> MGSSHHHHHHTGGTHPAVRVADLLQHINQMKTAEGYGFKQEYESFFEGWDATKKKDKVKGSRQEPMPAYDRHRVKLHPMLGDPSADYINANYIDGYHRSNHFIATQGPKPEMVYDFWRMVWQEHCSSIVMITKLVEVGRVKCSRYWPEDSDTYGDIKIMLVKTETLAEYVVRTFALERRGYSARHEVRQFHFTAWPEHGVPYHATGLLAFIRRVKASTPPDAGPIVIHCSAGTGRTGCYIVLDVMLDMAECEGVVDIYNCVKTLCSRRVNMIQTEEQYIFIHDAILEACLCGETTIP

PTPRU is a member of the R2B receptor family, which includes PTPRK, PTPRM and PTPRT, characterised by large extracellular domains that mediate homophilic interactions and tandem intracellular PTP domains. PTPRU possesses evolutionarily conserved sequence changes to key catalytic motifs including non-canonical WPD (WPE) and pTyr recognition loop sequences (GSRQ rather than KNRY), as well as a unique threonine in the PTP loop. Here, we demonstrate through biochemical and structural studies that PTPRU is unique amongst the receptor-linked protein tyrosine phosphatases (RPTPs) in possessing two pseudophosphatase domains. Despite lacking catalytic activity, PTPRU can recruit substrates of catalytically active paralogs supporting a model where PTPRU functions as a scaffold to compete for binding to protein substrates.

The overall fold of PTPRU-D1 closely resembles related phosphatase domains (RMSD of 1.0 Å2 over 237 Cα atoms with PTPRK). The most striking difference is the absence of an ordered pTyr recognition loop. The structure and sequence of this loop is well conserved across the PTPs, with the key tyrosine of the ‘KNRY’ motif creating an active site pocket deep enough to exclude pSer/Thr residues, whilst favourably stacking with the phenol ring of bound pTyr substrates. In the PTPRU crystal structure residues 904–925 encompassing the pTyr recognition loop region are disordered, resulting in almost complete loss of the pocket that would normally bind the pTyr substrate. The conformation of this loop is highly conserved in classical PTPs, but in PTPRU-D1 this loop is arranged such that the sidechain of T1089 is in close proximity to the active site cysteine (3.0 Å between T1089 OG1 and C1085 SG atoms, Fig. 2dii). The T1089 sidechain forms a hydrogen bond with the backbone amide of R1091 capping the adjacent helix. A threonine at this position in the PTP loop is unique to the PTPRU-D1 domain and the more common hydrophobic residues at this position (Ala, Val, and Ile) are not capable of forming an equivalent interaction. This new loop orientation blocks the catalytic cysteine and would directly interfere with pTyr binding. Residues C1121 to M1127 in PTPRU are not well ordered and challenging to build in a single, reliable conformation in the electron density suggesting it may adopt multiple conformations. In PTP1B this renders the enzyme inactive but is reversible upon reduction and is proposed to be a protective intermediate during redox-regulated inhibition. This conformation of the PTPRU-D1 PTP loop is not induced by oxidation, it is instead present in the reduced form rendering the enzyme unable to bind pTyr.> IVGGYTCAANSIPYQVSLNSGSHFCGGSLINSQWVVSAAHCYKSRIQVRLGEHNIDVLEGNEQFINAAKIITHPNFNGNTLDN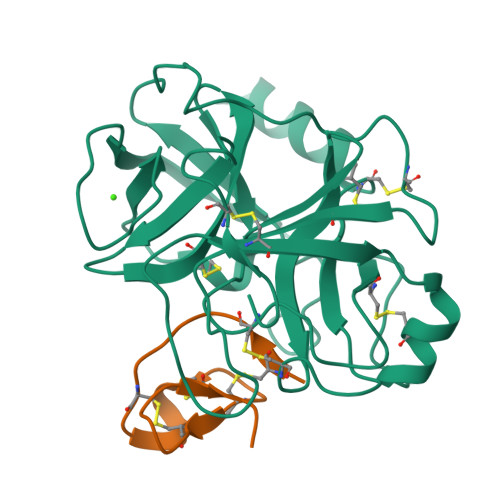DIMLIKLSSPATLNSRVATVSLPRSCAAAGTECLISGWGNTKSSGSSYPSLLQCLKAPVLSDSSCKSSYPGQITGNMICVGFLEGGKDSCQGDSGGPVVCNGQLQGIVSWGYGCAQKNKPGVYTKVCNYVNWIQQTIAAN;> GCPRILIRCKQDSDCLAGCVCTNNKFCGSPHHHHHH> MLRSTRPWRFRMKGGEMFVEYKIMSRDHRRSIRVEDAIVDPSVARTVVPLSWLEQLRSPSLRLHTGYHMEEAVYVPPAYAAVDEKEGRRLSEKSTMTPNAILAGPVVLSITGQSVPVVLNPYFVPDDTWGIRRNRDEWDLRLGMDAIEQCTLFSELRPGGLLYNKLPSSQNVTRHEPVRATLQRYGMKCGLAESPLVPRPWTRMRYMFIDELQRGPKLTEFVGHNPRNGTQWRFSQHSKYFRIGVWRETIRRNDMN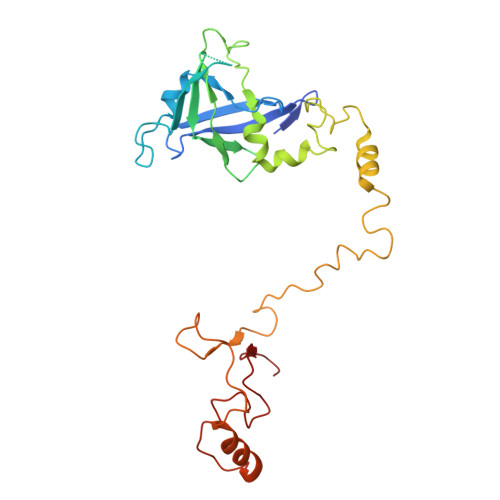EGLHGHSSWQKSPQQAVPEVRLMAPYP>HIERFEVVKRRAEMALHGNTVYIGGQVADDPSGDIQDQTRQILENIDRLLQSVGSDRGQVLSVRILLAHREDYAGLNQVWDQWFPEGRAPTRACSLAELIDPRWRVEMIVVAAREGHHHHHH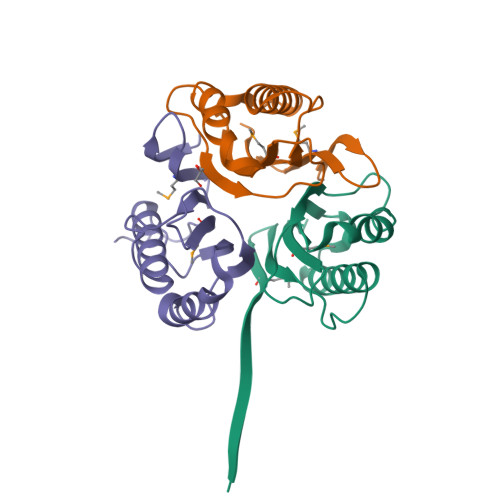[6x]>[2x]TRDQNGTWEMESNENFEGYMKALDIDFATRKIAVRLTQTLVIDQDGDNFKVKTTSTFFNYDVDFTVGVEFDEYTKSLDNRHVKALVTWEGDVLVCVQKGEKENRGWKKWIEGDKLYLELTCG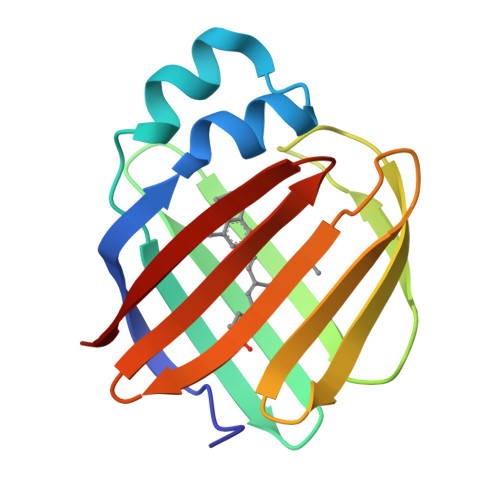DQVCRQVFKKK> ADVPAGVQLADKQTLVRNNGSEVQSLDPHKIEGVPESNVSRDLFEGLLISDVEGHPSPGVAEKWENKDFKVWTFHLRENAKWSDGTPVTAHDFVYSWQRLADPNTASPYASYLQYGHIANIDDIIAGKKPATDLGVKALDDHTFEVTLSEPVPYFYKLLVHPSVSPVPKSAVEKFGDKWTQPANIVTNGAYKLKNWVVNERIVLERNPQYWDNAKTVINQVTYLPISSEVTDVNRYRSGEIDMTYNNMPIELFQKLKKEIPNEVRVDPYLCTYYYEINNQKAPFNDVRVRTALKLALDRDIIVNKVKNQGDLPAYSYTPPYTDGAKLVEPEWFKWSQQKRNEEAKKLLAEAGFTADKPLTFDLLYNTSDLHKKLAIAVASIWKKNLGVNVNLENQEWKTFLDTRHQGTFDVARAGWCADYNEPTSFLNTMLSDSSNNTAHYKSPAFDKLIADTLKVADDTQRSELYAKAEQQLDKDSAIVPVYYYVNARLVKPWVGGYTGKDPLDNIYVKNLYI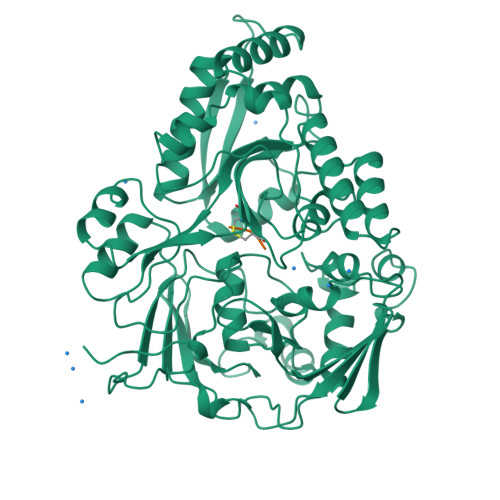IKH;> KCK>[2x]MSGTLMAFDFGTKSIGVAVGQRITGTARPLPAIKAQDGTPDWNIIERLLKEWQPDEIIVGLPLNMDGTEQPLTARARKFANRIHGRFGVEVKLHDERLSTVEARSGL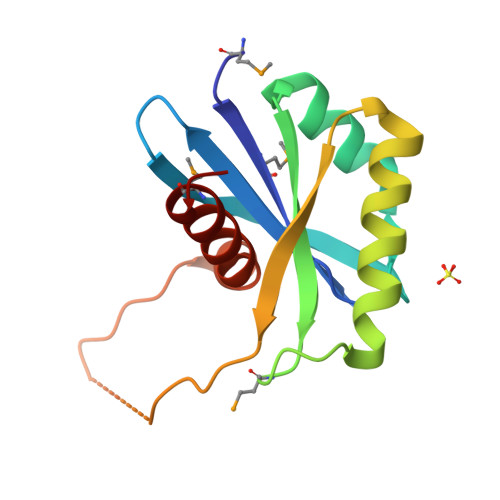FEQGGYRALNKGKVDSASAVIILESYMEQGY>KPYECYICHARFTQSGTMKMHILQKHTENVAKFHCPHCDTVIARKSDLGVHLRKQHSYIEQGKKCRYCDAVFHERYALIQHQKSHKNEKRFKCDQCDYASRQERHMIMHKRTHTGEKPYACSHCDKTFRQKQLL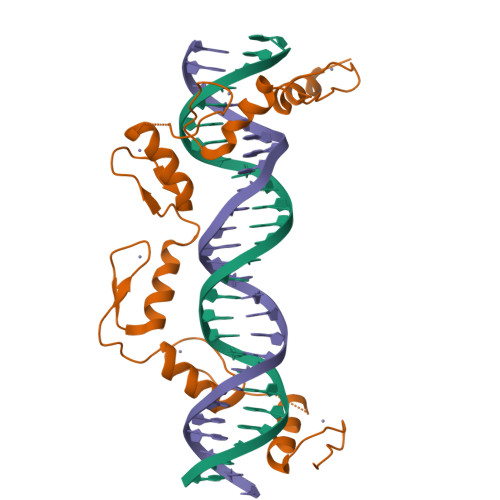DMHFKRYHDPNFVPAAFVCSKCGKTFTRRNTMARHADNCAGP[2x]>[2x]GHMAEVLVVTSKVKKLIKE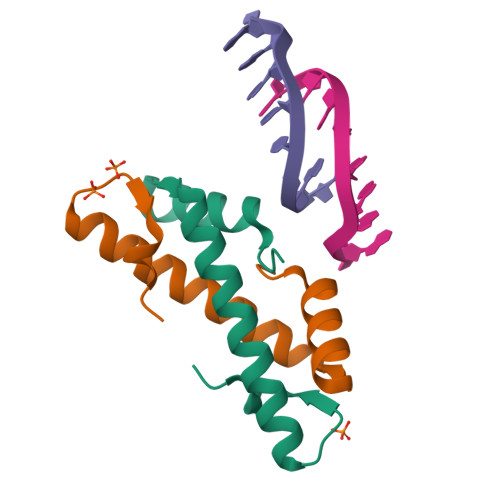KGQMNTSAETIDVLSKAIEQLCLKGVESAKADGRKTVMARDIVIDHL2-DEOXY-2,3-DEHYDRO-N-ACETYL-NEURAMINIC ACID | C11 H17 N O8 | 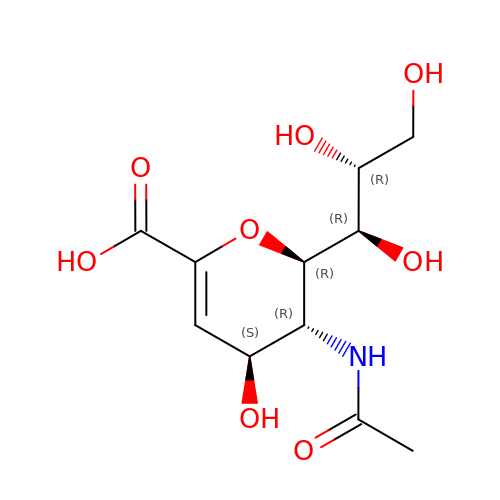JINJZWSZQKHCIP-UFGQHTETSA-N>MSAPVRVGVVGAGFMGGVHAEVVAAHPGARLEAVHDLDPAAARDLAERFRAERAEPSWADLLADPAIDLLIITTPNGLHHRQAAEALRAGKHVLVEKPLGVTPEQVAELVELAGRHDRVLAHGSNFVHSPKFVRARQLVADTEAFGRPHLVRVVFRNSGPEAAWAASKDLAGGGALLDLGCHAVELCRWLLDGADVESVSARLQRVRPPHDAEADRASGTAGTARVALEDQALLVMEFADGAVGQCDVSWVTQGGEQVTAEIIGTKGRVEVDLW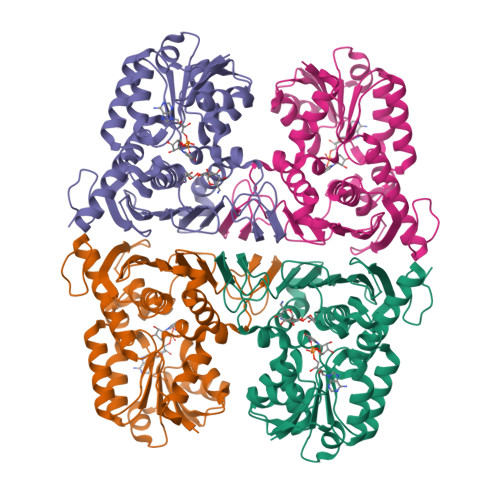TGMGLRAYSDKGYQDVWDPEQGWVHPEWEWIRASGYYHQDGTVIEAVGQGIPLTHGPAEALASARVLATGYRSHAEGRVLRLSGAPVGPGASTTAAGSEKLAAALEHHHHHH[2x]> EIGRTTDPVRMYMREMGTVELLTREGEIDIAKRIEDGINQVQCSVAEYPEAITYLLEQYDRVEAEEARLSDLITGFVDPNAEEDLAPTATHVGSELSQEDLDDDEDEDEEDGDDDSADDDNSIDPELAREKFAELRAQYVVTRDTIKAKGRSHATAQEEILKLSEVFKQFRLVPKQFDYLVNSMRVMMDRVRTQERLIMKLCVEQCKMPKKNFITLFTGNETSDTWFNAAIAMNKPWSEKLHDVSEEVHRALQKLQQIEEETGLTIEQVKDINRRMSIGEAKARRAKKEMVEANLRLVISIAKKYTNRGLQFLDLIQEGNIGLMKAVDKFEYRRGYKFSTYATWWIRQAITRSIADQARTIRIPVHMIETINKLNRISRQMLQEMGREPTPEELAERMLMPEDKIRKVLKIAKEPISMETPIGDDEDSHLGDFIEDTTLELPLDSATTESLRAATHDVLAGLTAREAKVLRMRFGIDMNTDYTLEEVGKQFDVTRERI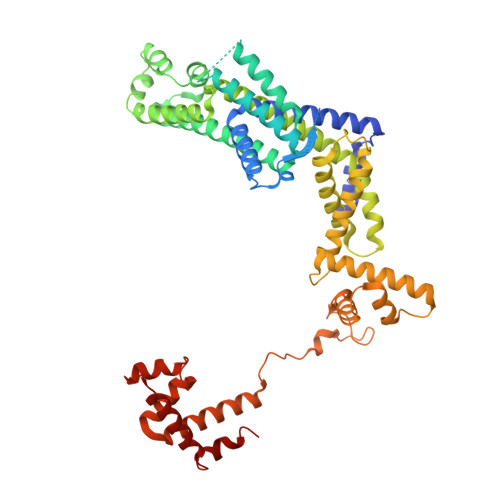RQIEAKALRKLRHPSRSEVLRSFLD GERANYL DIPHOSPHATE 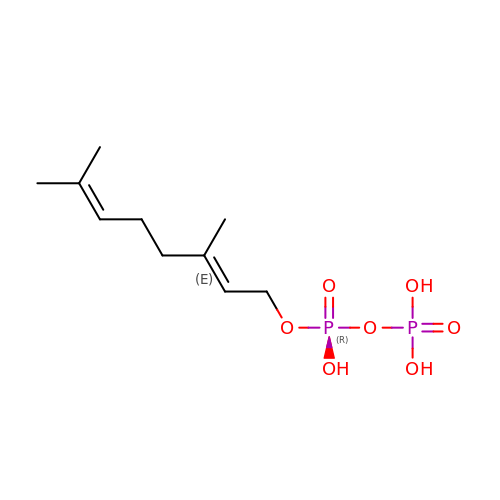| C10 H20 O7 P2 | GVVPGTZRZFNKDS-JXMROGBWSA-N> MTSLYAPGAEDIRQRLRPFGFFFEKSLKDLIKGIRSHNETPEKLDQFFKQVLSECREEVNSPDLNSKTNAVLKLTYLEMYGFDMAWCNFHILEVMSSNKLQQKRVGYLAASQSFYKDSDILMLATNLLKKDLKYDGNNDVVKVGIALSGLSTIITPSLARDIADDLFTMLNSTRPYIRKKAITALFKVFLQYPEALRDNFDKFVSKLDDDDISVVSAAVSVICELSKKNPQPFIQLSPLLYEILVTIDNNWIIIRLLKLFTNLSQVEPKLRAKLLPKILELMESTVATSVIYESVNCIVKGNMLEEDDFETAMACLERLHTFCDSQDPNLRYISCILFYKIGKINTDFISRFDQLIIRLLSDVDVSIRSKAIELVEGIVDEDNLKAIVQTLMKQFVDEDVVILQTGSIVYEKSKRIPIIIPENYKIKMVNVIISICSADNYSSVNDFEWYNAVIMDLAMLCQDISDKSLGSKIGEQFRNLMIKVPSMREVTIANIIKLISNDNINKQLPTVLRECIWCLGEFSTLVENGNDLIKIMTENISYYSHSVQEVLILALVKVFSNWCNNFQEDKRFEIKMVLKELIEFFENLSYSSTFEVQERSVEVLEFLRLSLEALEEDTEGLPMLLSEVLPSFFNAYELAPIARGTQLKLAVDENLDLETPFLTKEAADELLDEQKSDAISDLMSDISMDEQVELKFVDDSDTSYEEKEKLDDFENPFEIEREKERMSNPYYLGEEDEERTKNSKDLLDLNEEESSDKKPETIRLNRTDNSLNSLSLSTTEISRKKKKGKKKNRVQVLSDEPVIEAAPKRKDAFQKPHDNHSTQNPLKKDKINLRMHSQLENFDFSNFGQSSNAGRGSQEEGNLRKEDELELSRLEANLIVKDEKDNLSDTEEVIVIKKKKKGKKSKSKNKLKTKAKNSPEPNEFLRDQSTDIRTLQVDGSDYKDDDDKDYKDDDDKDYKDDDDK;> MVDSIHRIASALDTAKVITREAAAVATSKLGESSYTYYSQNINPQQLVTLLNSRNSREVRDAMKRIISIMASDDDSIDVQLYFADVVKNITTNDTKVKRLIHLYLLRFAENDPNLTLLSINSLQKSLSDSNSELRCFALSALSDMKMSSLAPIILHTVKKLVTDPSAMVRGEVALAIIKLYRAGKNDYHEELLDILKELMADTDPKVISCAVLAYKECYADHLELLHGHFRRYCRIIKQLDSWSQSYLIELLIKYCKQYLPKPTVVDKSSEGSPRSCPLPDKYNEIEYPSYEVVNDPDLDLFLQSLNCLIYSSNPTVILSCCNALYQLASPLQMKNTKFIEALVRTVTMTENQGNKEMLLQAIHFLSILDQTLFLPYTKKFYVFPKDPIVASIWKIQILSTLINESNVKEIFKELKYYVASAHFPENVVIMAVKSLSRCGQLSTSWESHVMKWLIDHMESHNLSASVLDAYVNVIRMLVQKNPTKHLRIIFKLADLLTVQTSLADNARAGIVWLFGEIASIEFKICPDVLRRLIQNFSNEGPETRCQILVLSA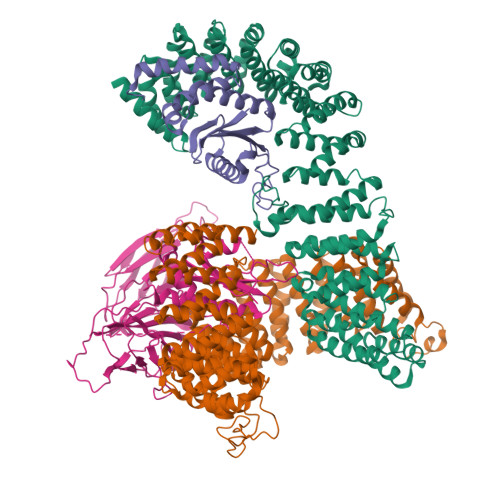KLLSYDIDNFKQAQVTGSEENNQNPPYYDFSGSRISQMYNAVLYLAKYDDEFDIRDRARMISSLFDSGKYEIVSLLLQAPKPTARSDDFIVSARLETHTPEIKEFFRMLPWNTEITEVGETGNDIREGAELKDYNKYKKSFSSQSFITNNSARSFTSSSNAKLTGINDGDSNSISGKGNVNTFTSQNGKKYRLQSLDEFFSDIPERKSKPRKIIKVVEESSDEDEDESEESSDDDEYSDSSLGTSSSGTSSSHLEL;> MYLSFYITDTKNKLIFQYLLGATAPSFKHLWTRVQSTCPQLLEDSSSDDYLDHSMVGRDLEVYKYFSVINKLNYWCLASTSKSKGPLDCFTFLETIDRILLEYFDKDKLSIKKIVNNYDRISLIFNCCVEAGEPNVSDMLYVNKIKEAVPERSDLSKFISSTAHNLQQAVQLPQQRQQQLQQNQISRGSNSLIENEEIVPWRTSRASKHENNELYVDLLETFHVVFEKKKSHLRLLTGSIHGIVDVRSYLNDNPLVAVKLNTMGNDIGIPSLHDCVEINDGVFSPSNITFIPPDGKFRLLEYSVDLSSQVKQSGVRMNSIGLMSLHFQNGLGKDSDEFELSLNIENFKKVSQVDDLKIDLQFNVENADPNEIAYKIKILRNTHGRFENSIIMGQGQWIFDKSTATGTVPVLRGCIEYENTGPNFTKKVDLQTVSLEYSYIGQSASGIYVEAIDIVSGLTIGKNTKLYKGAKYKTQTGNFQVRL;> MIHAVLIFNKKCQPRLVKFYTPVDLPKQKLLLEQVYELISQRNSDFQSSFLVTPPSLLLSNENNNDEVNNEDIQIIYKNYATLYFTFIVDDQESELAILDLIQTFVESLDRCFTEVNELDLIFNWQTLESVLEEIVQGGMVIETNVNRIVASVDELNKAAESTDSKIGRLTSTGFGSALQAFAQGGFAQWATGQ2-[2-[carboxymethyl-[(2-hydroxyphenyl)methyl]amino]ethyl-[(2,3-dihydroxyphenyl)methyl]amino]ethanoic acid | C20 H24 N2 O7 | 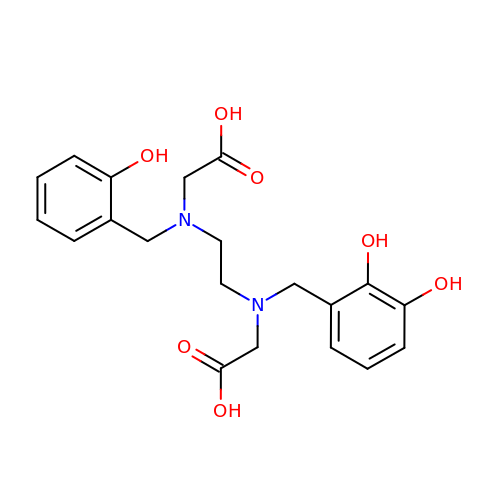PIRBWSIWJQHRSO-UHFFFAOYSA-N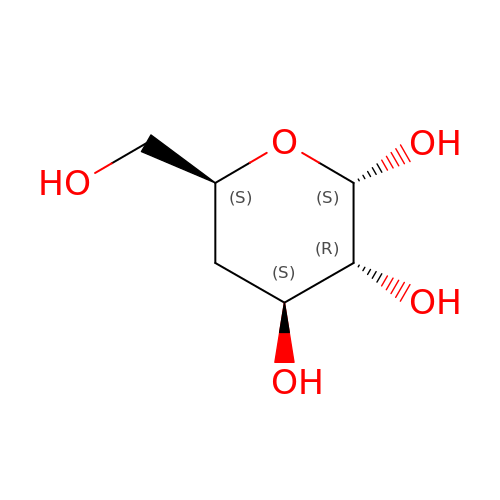4-deoxy-alpha-D-glucopyranose | C6 H12 O5 | HDEMQQHXNOJATE-AZGQCCRYSA-N>MKKRLTITLSESVLENLEKMAREMGLSKSAMISVALEN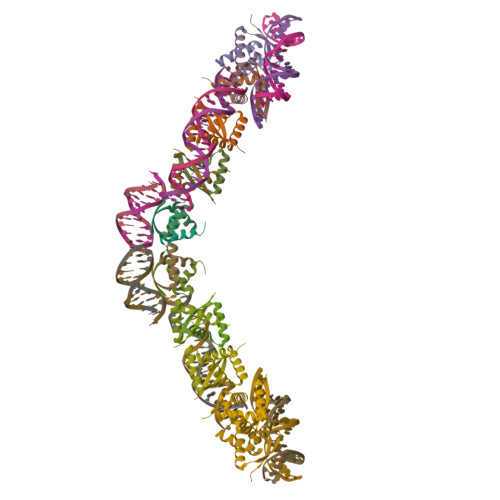YKKGQEK[10x]> PISPIETVPVKLKPGMDGPKVKQWPLTEEKIKALVEICTEMEKEGKISKIGPENPYNTPVFAIKKKDSTKWRKLVDFRELNKRTQDFWEVQLGIPHPAGLKKKKSVTVLDVGDAYFSVPLDEDFRKYTAFTIPSINNETPGIRYQYNVLPQGWKGSPAIFQSSMTKILEPFKKQNPDIVIYQYMDDLYVGSDLEIGQHRTKIEELRQHLLRWGLTTPDKKHQKEPPFLWMGYELHPDKWTVQPIVLPEKDSWTVNDIQKLVGKLNWASQIYPGIKVRQLCKLLRGTKALTEVIPLTEEAELELAENREILKEPVHGVYYDPSKDLIAEIQKQGQGQWTYQIYQEPFKNLKTGKYARMRGAHTNDVKQLTEAVQKITTESIVIWGKTPKFKLPIQKETWETWWTEYWQATWIPEWEFVNTPPLVKLWYQLEKEPIVGAETFYVDGAANRETKLGKAGYVTNKGRQKVVPLTNTTNQKTELQAIYLALQDSGLEVNIVTDSQYALGIIQAQPDKSESELVNQIIEQLIKKEKVYLAWVPAHKGIGGNEQVDKLVSAGI;> PISPIETVPVKLKPGMDGPKVKQWPLTEEKIKALVEICTEMEKEGKISKI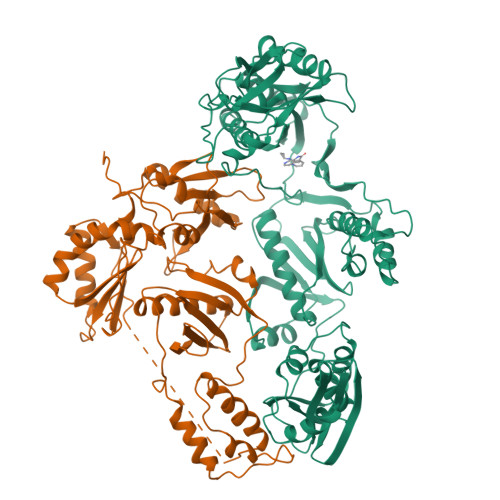GPENPYNTPVFAIKKKDSTKWRKLVDFRELNKRTQDFWEVQLGIPHPAGLKKKKSVTVLDVGDAYFSVPLDEDFRKYTAFTIPSINNETPGIRYQYNVLPQGWKGSPAIFQSSMTKILEPFKKQNPDIVIYQYMDDLYVGSDLEIGQHRTKIEELRQHLLRWGLTTPDKKHQKEPPFLWMGYELHPDKWTVQPIVLPEKDSWTVNDIQKLVGKLNWASQIYPGIKVRQLCKLLRGTKALTEVIPLTEEAELELAENREILKEPVHGVYYDPSKDLIAEIQKQGQGQWTYQIYQEPFKNLKTGKYARMRGAHTNDVKQLTEAVQKITTESIVIWGKTPKFKLPIQKETWETWWTEYWQATWIPEWEFVNTPPLVKLWYQ methyl (~{Z})-3-(4-acetamidophenyl)-2-methyl-prop-2-enoate 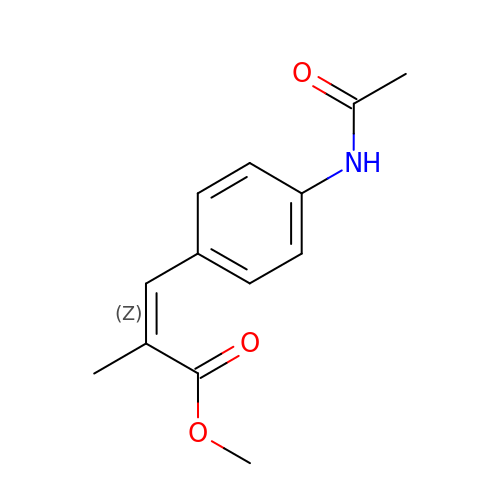| C13 H15 N O3 | UPZAERQJNSXZQO-HJWRWDBZSA-N> MYVYKRDGRKEPVQFDKITARISRLCYGLDPKHIDAVKVTQRIISGVYEGVTTIELDNLAAETCAYMTTVHPDYATLAARIAISNLHKQTTKQFSKVVEDLYRYVNAATGKPAPMISDDVYNIVMENKDKLNSAIVYDRDFQYSYFGFKTLERSYLLRINGQVAERPQHLIMRVALGIHGRDIEAALETYNLMSLKYFTHASPTLFNAGTPKPQMSSCFLVAMKEDSIEGIYDTLKECALISKTAGGIG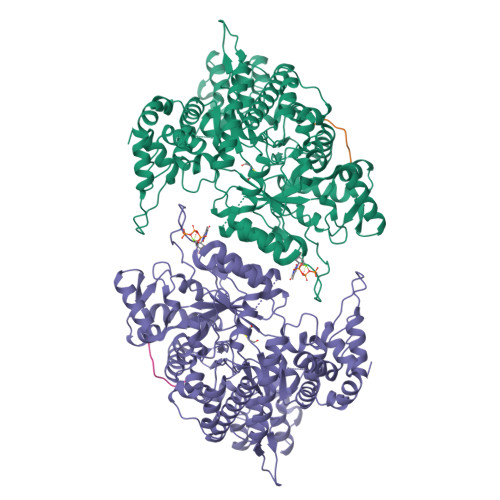LHIHNIRSTGSYIAGTNGTSNGLIPMIRVFNNTARYVDQGGNKRPGAFALYLEPWHADIFDFIDIRKNHGKEEIRARDLFPALWIPDLFMKRVEENGTWTLFSPTSAPGLSDCYGDEFEALYTRYEKEGRGKTIKAQKLWYSILEAQTETGTPFVVYKDACNRKSNQKNLGVIKSSNLCCEIVEYSAPDETAVCNLASVALPAFIETSEDGKTSTYNFKKLHEIAKVVTRNLNRVIDRNYYPVEEARKSNMRHRPIALGVQGLADTFMLLRLPFDSEEARLLNIQIFETIYHASMEASCELAQKDGPYETFQGSPASQGILQFDMWDQKPYGMWDWDTLRKDIMKHGVRNSLTMAPMPTASTSQILGYNECFEPVTSNMYSRRVLSGEFQVVNPYLLRDLVDLGIWDEGMKQYLITQNGSIQGLPNVPQELKDLYKTVWEISQKTIINMAADRSVYIDQSHSLNLFLRAPTMGKLTSMHFYGWKKGLKTGMYYLRTQAASAAIQFTIDQKIADQATENVADISNLKRPSYMPSSASYAASDFVPAAVTANATIPSLDSSSEASREASPAPTGSHSLTKGMAELNVQESKVEVPEVPAPTKNEEKAAPIVDDEETEFDIYNSKVIACAIDNPEACEMCSG;> GAFTFNEDF> MIIPALDLIDGTVVRLHQGDYARQRDYGNDPLPRLQDYAAQGAGVLHLVDLTGAKDPAKRQIPLIKTLVAGVNVPVQVGGGVRTEEDVAALLKAGVARVVIGSTAVKSPDVVK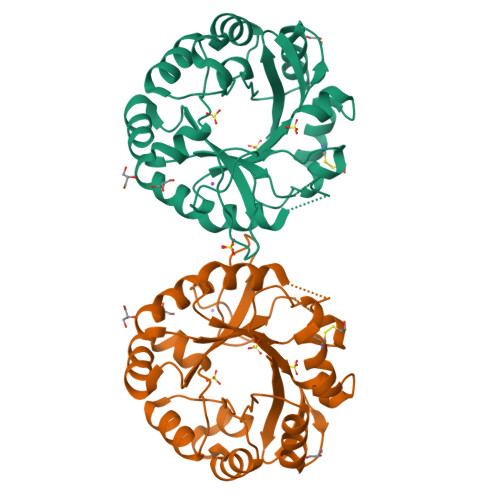GWFERFGAQALVLALDVRIDEHGTKQVAVSGWQENSGVSLEQLVETYLPVGLKHVRCTDISRDGTLAGSNVSLYEEVCARYPQIAFQSSGGIGDIDDIAALRGTGVRGVIVGRALLEGKFTVKEAIQCWQNVKGHHHHHH>MAVPSLWPWGACLPVIFLSLGFGLDTVEVCPSLDIRSEVAELRQLENCSVVEGHLQILLMFTATGEDFRGLSFPRLTQVTDYLLLFRVYGLESLRDLFPNLAVIRGTRLFLGYALVIFEMPHLRDVALPALGAVLRGAVRVEKNQELCHLSTIDWGLLQPAPGANHIVGNKLGEECADVCPGVLGAAGEPCAKTTFSGHTDYRCWTSSHCQRVCPCPHGMACTARGECCHTECLGGCSQPEDPRACVACRHLYFQGACLWACPPGTYQYESWRCVTAERCASLHSVPGRASTFGIHQGSCLAQCPSGFTRNSSSIFCHKCEGLCPKECKVGTKTIDSIQAAQDLVGCTHVEGSLILNLRQGYNLEPQLQHSLGLVETITGFLKIKHSFALVSLGFFKNLKLIRGDAMVDGNYTLYVLDNQNLQQLGSWVAAGLTIPVGKIYFAFNPRLCLEHIYRLEEVTGTRGRQNKAEINPRTNGDRAACQTRTLRFVSNVTEADRILLRWERYEPLEARDLLSFIVYYKESPFQNATEHVGPDACGTQSWNLLDVELPLSRTQEPGVTLASLKPWTQYAVFVRAITLTTEEDSPHQGAQSPIVYLRTLPAAPTVPQDVISTSNSSSHLLVRWKPPTQRNGNLTYYLVLWQRLAEDGDLYLNDYCHRGLRLPTSNNDPRFDGEDGDPEAEMESDCCPCQHPPPGQVLPPLEAQEASFQKKFENFLHNAITIPISPWKVTSINKSPQRDSGRHRRAAGPLRLGGNSSDFEIQEDKVPRERAVLSGLRHFTEYRIDIHACNHAAHTVGCSAATFVFARTMPHREADGIPGKVAWEASSKNSVLLRWLEPPDPNGLILKYEIKYRRLGEEATVLCVSRLRYAKFGGVHLALLPPGNYSARVRATSLAGNGSWTDSVAFYILGPEEEDAGGLHVLLTATPVGLTLLIVLAALGFFYGKKRNRTLYASVNPEYFSASDMYVPDEWEVPREQISIIRELGQGSFGMVYEGLARGLEAGEESTPVALKTVNELASPRECIEFLKEASVMKAFKCHHVVRLLGVVSQGQPTLVIMELMTRGDLKSHLRSLRPEAENNPG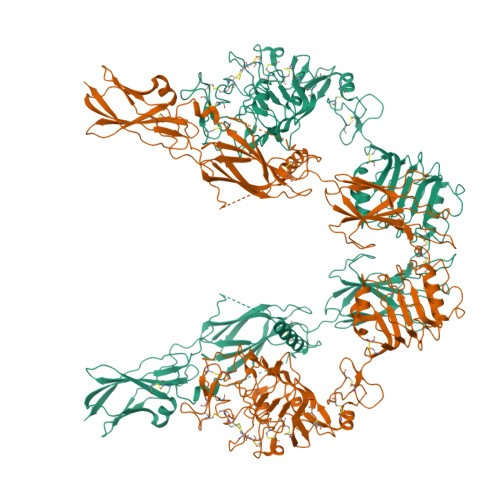LPQPALGEMIQMAGEIADGMAYLAANKFVHRDLAARNCMVSQDFTVKIGDFGMTRDVYETDYYRKGGKGLLPVRWMAPESLKDGIFTTHSDVWSFGVVLWEIVTLAEQPYQGLSNEQVLKFVMDGGVLEELEGCPLQLQELMSRCWQPNPRLRPSFTHILDSIQEELRPSFRLLSFYYSPECRGARGSLPTTDAEPDSSPTPRDCSPQNGGPGH[2x]>DGWNKLFDLIQSELYVRPDDVHVNIRLVEVYRSTKRLKDAVAHCHEAERNIALRSSLEWNSCVVQTLKEYLESLQCLESDKSDWRATNTDLLLAYANLMLLTLSTRDVQESRELLQSFDSALQSVKSLGGNDELSATFLEMKGHFYMHAGSLLLKMGQHSSNVQWRALSELAALCYLIAFQVPRPKI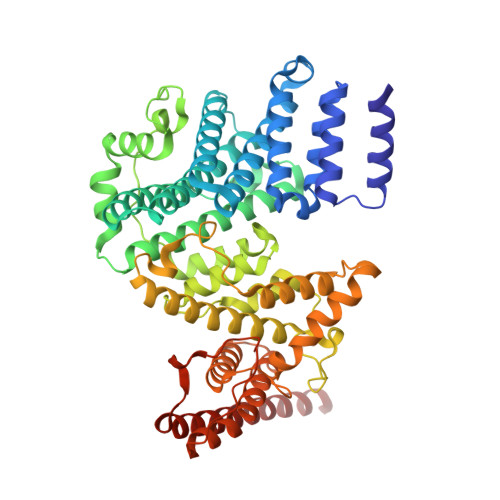KLIKGEAGQNLLEMMACDRLSQSGHMLLNLSRGKQDFLKEIVETFANKSGQSALYDALFSSQSPKDTSFLGSDDIGNIDVREPELEDLTRYDVGAIRAHNGSLQHLTWLGLQWNSLPALPGIRKWLKQLFHHLPHETSRLETNAPESICILDLEVFLLGVVYTSHLQLKEKCNSHHSSYQPLCLPLPVCKQLCTERQKSWWDAVCTLIHRKAVPGNVAKLRLLVQHEINTLRAQEKHGLQPALLVHWAECLQKTGSGLNSFYDQREYIGRSVHYWKKVLPLLKIIKKKNSIPEPIDPLFKHFHSVDIQASEIVEYEEDAHITFAILDAVNGNIEDAVTAFES[3x]> MKLDIKKTFSNRSDRVKGIDFHPTEPWVLTTLYSGRVELWNYETQVEVRSIQVTETPVRAGKFIARKNWIIVGSDDFRIRVFNYNTGEKVVDFEAHPDYIRSIAVHPTKPYVLSGSDDLTVKLWNWENNWALEQTFEGHEHFVMCVAFNPKDPS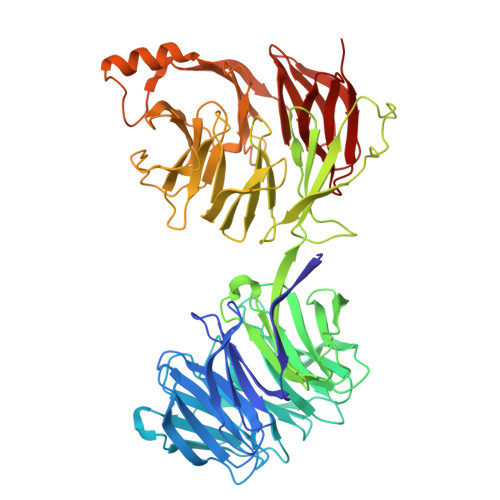TFASGCLDRTVKVWSLGQSTPNFTLTTGQERGVNYVDYYPLPDKPYMITASDDLTIKIWDYQTKSCVATLEGHMSNVSFAVFHPTLPIIISGSEDGTLKIWNSSTYKVEKTLNVGLERSWCIATHPTGRKNYIASGFDNGFTVLSLGNDEPTLSLDPVGKLVWSGGKNAAASDIFTAVIRGNEEVEQDEPLSLQTKELGSVDVFPQSLAHSPNGRFVTVVGDGEYVIYTALAWRNKAFGKCQDFVWGPDSNSYALIDETGQIKYYKNFKEVTSWSVPMHSAIDRLFSGALLGVKSDGFVYFFDWDNGTLVRRIDVNAKDVIWSDNGELVMIVNTNSNGDEASGYTLLFNKDAYLEAANNGNIDDSEGVDEAFDVLYELSESITSGKWVGDVFIFTTATNRLNYFVGGKTYNLAHYTKEMYLLGYLARDNKVYLADREVHVYGYEISLEVL>[2x]MP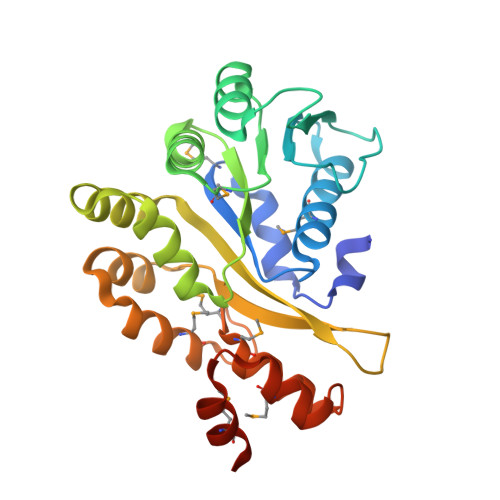AEIPEFKKLGLPDKVLELCHRKMGLILVTGPTGSGKSTTIASMIDYINQTKSYHIITIEDPIEYVFKHKKSIVNQREVGEDTKSFADALRAALREDPDVIFVGEMRDLETVETALRAAETGHLVFGTLHTNTAIDTIHRIVDIFPLNQQEQVRIVLSFILQGIISQRLLPKIGGGRVLAYGLLIPNTAIRNLIRENKLQQVYSLMQSGQAETGMQTMNQTLYKLYKQGLITLEDAMEASPDPKELERMIRGGRHHHHHH> GAMDQVQLIKRKDSGRYEIVPIEDPLSFEKGFYAVIRACQLLAQKNDGLILVGLAGPSGAGKTIFTEKILNFMPSIAIINMDNYNDGTRVIDGNFDDPRLTDYDTLLDNIHGLRDGKPVQVPIYDFKSSSRIGYRTLEVPSSRIVILEGIYALSEKLRPLLDLRVSVTGGVHFDLVKRVLRDIQRAGQEPEEIIHQISETVYPMYKAFIEPDLKTAQIKILNKFNPFSGFQNPTYILKSSKAVTPEQMKAALSEDFKERTEETYDIYLLPPGE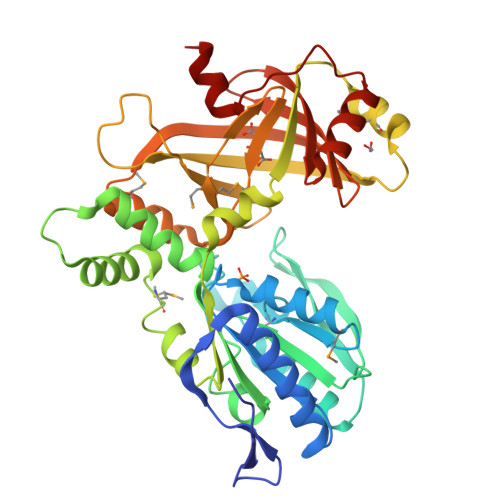DPEACQSYLRMRNRDGKYNLMFEEWVTDRPFIISPRITFEVSVRLLGGLMALGYTIATILKRKSHIFDDDKVIVKTDWLEQLNRTYVQVQGKDRTFVKNVADQLGLEGSYVPHTYIEQIQLER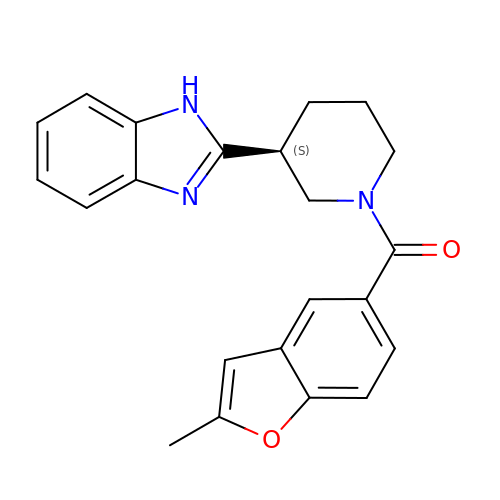[(3S)-3-(1H-benzimidazol-2-yl)piperidin-1-yl](2-methyl-1-benzofuran-5-yl)methanone | C22 H21 N3 O2 | PWUXNVBUFJIXEG-INIZCTEOSA-N>MRLLHTM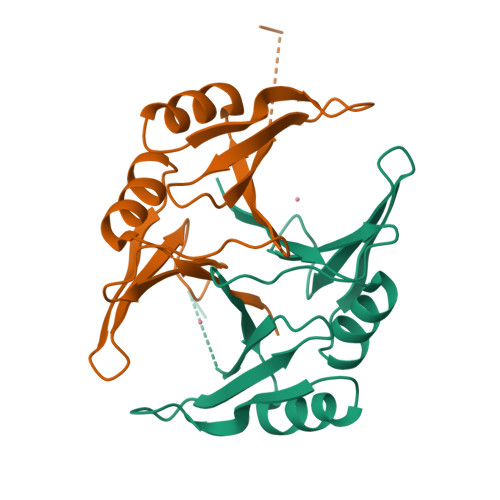LRVGDLQRSIDFYTKVLGMKLLRTSENPEYKYSLAFVGYGPETEEAVIELTYNWGVDKYELGTAYGHIALSVDNAAEACEKIRQNGGNVTREAGPVKGGTTVIAFVEDPDGYKIELIEEKDAGRGLGN[2x]>[2x]MFTGSIVAIVTPMDEKGNVCRASLKKLIDYHVASGTSAIVSVGTTGESATLNHDEHADVVMMTLDLADGRIPVIAGTGANATAEAISLTQRFNDSGIVGCLTVTPYFNRPSQEGLYQHFKAIAEHTDLPQ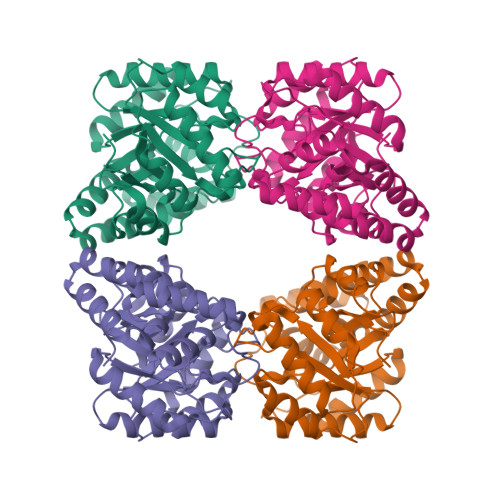ILYNVPSRTGCDLLPETVGRLAKVKNIIGIKEATGNLTRVNQIKELVSDDFVLLSGDDASALDFMQLGGHGVISVTANVAARDMAQMCKLAAEGHFAEARVINQRLMPLHNKLFVEPNPIPVKWACKELGLVATDTLRLPMTPITDSGRETVRAALKHAGLL> MGSDYKDDDDKSGMDNKLKTENIRYFRTAAGSEDVLEVKAYEVYPNVWAIPSRYMMEPLQDLDEVTNPEQFSIYDKKYLADIQEQDEFLKSIQAAIEDIKKRTFGLELLTAVSGAVPLPKDTGATNTTLQCIDENGKHTHDVVANVVLWGPGNNLNSNRLISKSDDDSNGIGSMVELIWNPQILIKNIGTNRIKPATDELVGLLTKALFRLYGLGLNKIRYPFYQLDDKKYYSLTAEDLISYGGFSANVVNLQPYYFLEDQFTKVKEKYESAKKRIDDIKVNDEYSQMLTLKYQFDLYSLFHISTSYIVSTVIPANDKYGGLVSYYTGPNALIDSKTDEKLTSMVKIPLKKIKYSKNQSREYDEYDLTNGEDSTQYFENFTFPKSKHVFVETQPTPENVFVNLPSEEITKIILPVIPAESDLIKIPFQPATPKSITTELITTDVPTLGLIFPAVKSKQNLSDIKMTSKLSDALDSDKQTFAFDNTLVDKLSELTSVSDAELFGIIRLIKNELLSVIDNFTTFGDNWSCPRWIDYCFQQVFGSDLKNLIVQGDFEKVFNISDTLILPKQLPEDILQLKPYLFYQWYAKRYTRILRLESLFYQILNEHITLIRSLVSSNNKGQYLQGFMNDLDKIAYNAQYMLSDWTIQLGYYDFKNQVTQVIKTSSMTSEFNIDDLLYDYDTFKLTISQFGADSINNFTPSQDLKLALNDNNSPILLLGNDEIKSNGSITQTDDSLDDETSLLLSKNTSFEGNFSAKYLLSSVGVNFTFKSIENLNFSVDFMNINIAFSNNFFEITQTGQETKKYSIAKLFGWNSLVYLIKHSSVEIWDIHSNILLVSHDLTAPQNNIVKAPIKLTNLDNELILKSFEVFEQDEEANYNDIEQGFKNGIIYTAKKMPIIVGEKYALKSSILDDMGILTSDENKKYPVFSTDVEVESSLNIILESTTGDKISVDAGVNIRTINSNGEENYLGIEDNHLIFVPK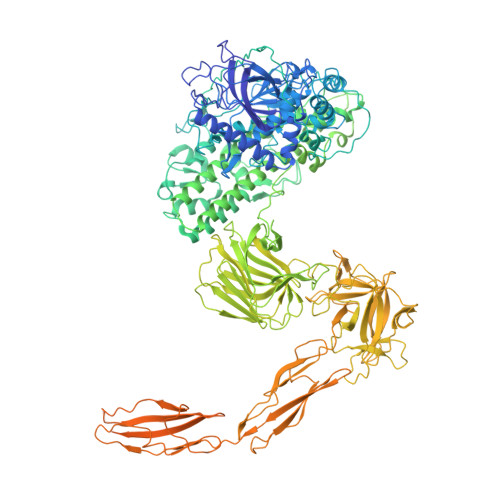EEAELFYLKKAVVEDTIDIFYVVKTLGNMFINVERISDNIYRLNFKAGILYSTMESDMLVLPAEEANTAFYIQPIGLASLEVKDSVLGEGNPWLKEDNFLDATDDYGNQIDLSDNRISVTGSVDTDKVGTYSVVYSYTGIDKTNTEKATITVKLDKSSIKTQDSTLQNGKEWVRADNLVEVIDEDGNKVDYSDDRIIQEGDVDINKAGVYDITFRYRGKFKIISSSFKVTVINDIWYDSIKNACKTYLIDYGERINDVKGITFQNILEATRGKLYGYRVVYDNPHDVINQNPPKDFHFDLIKPFDVKNPSRVHLADYSGYLRLFIISTGKINTDIKVKIYAVLENKDEIEIFDNHQNDKRHEEIAEIYKSNFDDNNYSADGKYFISVLFKNDVQAVVKDEIYGYEIFYSYFTKFRKDTAFQTDGSKRIFFHDYFNFEVPLDYKDSTFINVILKNGEKIRIYKFAGYYYYSGHHHHHH> MVQSMTSVVKAANFILARPTLSKIITPLAQKFTAYA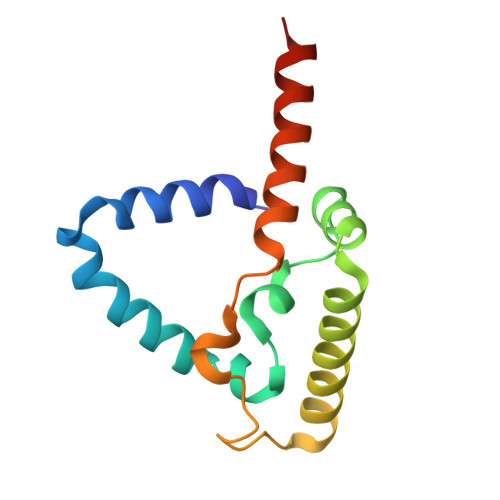GYREMGLKFNDLLLEETPIMQTAIKRLPSELNYSRNFRILTAHQLALSHQLLPAEKAVKPEEDDNYLIPYILEAEKEAFEKAELDNIEVKA> MGFFDRLKAGLAKTRERLLKAIPWGGNLEEVLEELEMALLAADVGLSATEEILQEVRASGRKDLKEAVKEKLVGMLEPDERRATLRKLGFNPQKPKPVEPKGRVVLVVGVNGVGKTTTIAKLGRYYQNLGKKVMFCAGDTFRAAGGTQLSEWGKRLSIPVIQGPEGTDSAALAYDAVQAMKARGYDLLFVDTAGRLHTKHNLMEELKKVKRAIAKADPEEPKEVWLVLDAVTGQ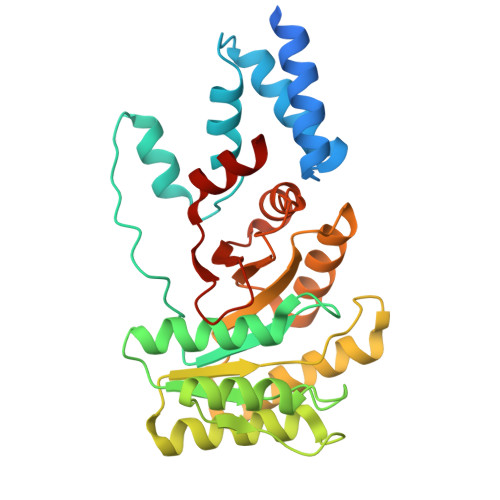NGLEQAKKFHEAVGLTGVIVTKLDGTAKGGVLIPIVRTLKVPIKFVGVGEGPDDLQPFDPEAFVEALLED> MSILTRWLLIPPVNARLIGRYRDYRRHGASAFSATLGCFWMILAWIFIPLEHPRWQRIRAEHKNLYPHINASRPRPLDPVRYLIQTCWLLIGASRKETPKPRRRAFSGLQNIRGRYHQWMNELPERVSHKTQHLDEKKELGHLSAGARRLILGIIVTFSLILALICVTQPFNPLAQFIFLMLLWGVALIVRRMPGRFSALMLIVLSLTVSCRYIWWRYTSTLNWDDPVSLVCGLILLFAETYAWIVLVLGYFQVVWPLNRQPVPLPKDMSLWPSVDIFVPTYNEDLNVVKNTIYASLGIDWPKDKLNIWILDDGGREEFRQFAQNVGVKYIARTTHEHAKAGNINNALKYAKGEFVSIFDCDHVPTRSFLQMTMGWFLKEKQLAMMQTPHHFFSPDPFERNLGRFRKTPNEGTLFYGLVQDGNDMWDATFFCGSCAVIRRKPLDEIGGIAVETVTEDAHTSLRLHRRGYTSAYMRIPQAAGLATESLSAHIGQRIRWARGMVQIFRLDNPLTGKGLKFAQRLCYVNAMFHFLSGIPRLIFLTAPLAFLLLHAYIIYAPALMIALFVLPHMIHASLTNSKIQGKYRHSFWSEIYETVLAWYIAPPTLVALINPHKGKFNVTAKGGLVEEEYVDWVISRPYIFLVLLNLVGVAVGIWRYFYGPPTEMLTVVVSMVWVFYNLIVLGGAVAVSVESKQVRRSHRVEMTMPAAIAREDGHLFSCTVQDFSDGGLGIKINGQAQILEGQKVNLLLKRGQQEYVFPTQVARVMGNEVGLKLMPLTTQQHIDFVQCTFARADTWALWQDSYPEDKPLESLLDILKLGFRGYRHLAEFAPSSVKGIFRVLTSLVSWVVSFIPRRPERSETAQPSDQALAQQGSARSSGRTGLEFEEFYPYDVPDYAADYKDDDDKRS;> TPATQPLINAEPAVAAQTEQNPQVGQVMPGVQGADAPVVAQNGPSRDVKLTFAQIAPPPGSMVLRGINPNGSIEFGMRSDEVVTKAMLNLEYTPSPSLLPVQSQLKVYLNDELMGVLPVTKEQLGKKTLAQMPINPLFITDFNRVRLEFVGHYQDVCENPASTTLWLDVGRSSGLDLTYQTLNVKNDLSHFPVPFFDPRDNRTNTLPMVFAGAPDVGLQQASAIVASWFGSRSGWRGQNFPVLYNQLPDRNAIVFATNDKRPDFLRDHPAVKAPVIEMINHPQNPYVKLLVVFGRDDKDLLQAAKGIAQGNILFRGESVVVNEVKPLLPRKPYDAPNWVRTDRPVTFGELKTYEEQLQSSGLEPAAINVSLNLPPDLYLMRSTGIDMDINYRYTMPPVKDSSRMDISLNNQFLQSFNLSSKQEANRLLLRIPVLQGLLDGKTDVSIPALKLGATNQLRFDFEYMNPMPGGSVDNCITFQPVQNHVVIGDDSTIDFSKYYHFIPMPDLRAFANAGFPFSRMADLSQTITVMPKAPNEAQMETLLNTVGFIGAQTGFPAINLTVTDDGSTIQGKDADIMIIGGIPDKLKDDKQIDLLVQATESWVKTPMRQTPFPGIVPDESDRAAETRSTLTSSGAMAAVIGFQSPYNDQRSVIALLADSPRGYEMLNDAVNDSGKRATMFGSVAVIRESGINSLRVGDVYYVGHLPWFERLWYALANHPILLAVLAAISVILLAWVLWRLLRIISRRRLNPDNE;>[3x]MTQFTQNTAMPSSLWQYWRGLSGWNFYFLVKFGLLWAGYLNFHPLLNLVFAAFLLMPLPRYSLHRLRHWIALPIGFALFWHDTWLPGPESIMSQGSQVAGFSTDYLIDLVTRFINWQMIGAIFVLLVAWLFLSQWIRITVFVVAILLWLNVLTLAGPSFSLWPAGQPTTTVTTTGGNAAATVAATGGAPVVGDMPAQTAPPTTANLNAWLNNFYNAEAKRKSTFPSSLPADAQPFELLVINICSLSWSDIEAAGLMSHPLWSHFDIEFKNFNSATSYSGPAAIRLLRASCGQTSHTNLYQPANNDCYLFDNLSKLGFTQHLMMGHNGQFGGFLKEVRENGGMQSELMDQTNLPVILLGFDGSPVYDDTAVLNRWLDVTEKDKNSRSATFYNTLPLHDGNHYPGVSKTADYKARAQKFFDELDAFFTELEKSGRKVMVVVVPEHGGALKGDRMQVSGLRDIPSPSITDVPVGVKFFGMKAPHQGAPIVIEQPSSFLAISDLVVRVLDGKIFTEDNVDWKKLTSGLHKQHRSPRTQMQ

Bacterial cellulosic polymers constitute a prevalent class of biofilm matrix exopolysaccharides that are synthesized by several types of bacterial cellulose secretion (Bcs) systems, which include conserved cyclic diguanylate (c-di-GMP)-dependent cellulose synthase modules together with diverse accessory subunits. In E. coli, the biogenesis of phosphoethanolamine (pEtN)-modified cellulose relies on the BcsRQABEFG macrocomplex, encompassing inner-membrane and cytosolic subunits, and an outer membrane porin, BcsC. Here we present cryo-EM structures of the E. coli Bcs macrocomplex positioning all seven BcsRQABEFG partners and multiple c-di-GMP-binding sites.

We show that the Bcs macrocomplex contains a single BcsA synthase, which associates in the membrane with hexameric BcsB on one side and a trimeric BcsG pEtN-transferase complex on the other. Indeed, using local refinement to resolve the more dynamically associated pEtN-transferase, we show here that BcsANTD adopts an amphipathic fold and recruits three copies of the BcsG pEtN-transferase whose transmembrane N-terminal domains are tightly packed between BcsATMD and the sixth BcsB protomer of the crown, whereas the C-terminal catalytic BcsG modules remain unresolved in the structures. The BcsA N-terminus folds into a W-shaped series of amphipathic α–helices whose connecting loops coordinate the BcsG protomers via conserved amino acid motifs in an otherwise weakly conserved primary structure. The first and second BcsB copies engage in contacts with the BcsA synthase, where the C-terminal TA of BcsB1 fits in a groove formed by BcsA TMα1–3 and is further encased by BcsANTD to complete the membrane export module, while BcsB2-TA engages in limited hydrophobic contacts with the loop connecting BcsA TMα3 and TMα4 at the periplasmic side of the inner membrane. Interestingly, in BcsG the amphipathic helical loops point outwards relative to the crown’s lumen, where BcsB’s stacked carbohydrate-binding domains are proposed to form the polysaccharide extrusion path. This suggests major conformational gymnastics of the catalytic C-terminal domains for pEtN extraction and transfer onto the nascent cellulosic polymer, and could potentially explain the lack of resolved BcsGCTD-corresponding regions in the averaged electron density maps. Consistent with our earlier but indirect BACTH results, we reveal here that the E. coli-like BcsA synthases have evolved a specific N-terminal amphipathic domain, whose W-shaped fold recruits three copies of the BcsG pEtN-transferase. On the other side of the β-barrel, an intercalated c-di-GMP dimer is found coordinated between the arginines from the canonical R696RxxR motif in the N-proximal PilZ domain linker, the active site gating loop is unstructured, and the active site is substrate-accessible.>ASNAPAPLAGVIFEPFQELKKDYLAVPIAHNVSLARQNYADDSESAINEQINVEYNVSYVYHALFAYFDRDNIALKGLA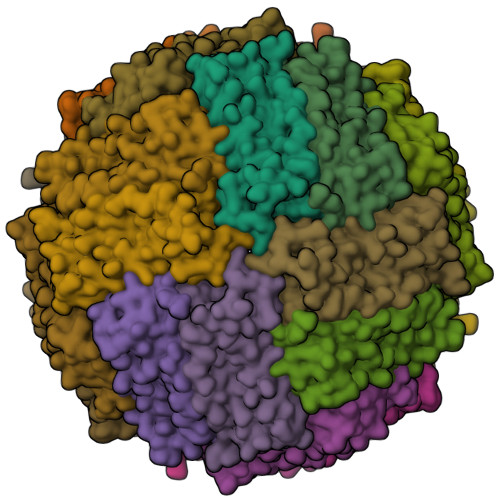KFFKESSEEEREHAEQLIKYQNIRGGRVVLHPITSPPSEFEHSEKGDALYAMELALSLEKLTNEKLLHVHSVADRNNDPQLADFIESEFLYEQVKSIKKIAEYVAQLRLVGKGHGVWHFDQKLLHDEDHV[6x]3-(aminomethyl)-4-(2,4-dichlorophenyl)-6-(2-methoxyethyl)-2-methyl-6,7-dihydro-5H-pyrrolo[3,4-b]pyridin-5-one 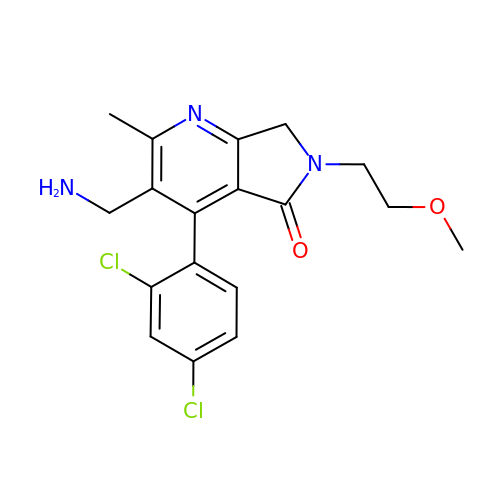| C18 H19 Cl2 N3 O2 | LKKWOSVPEMTNNP-UHFFFAOYSA-N> MGHHHHHHSHMAEIGTGFPFDPHYVEVLGERMHYVDVGPRDGTPVLFLHGNPTSSYVWRNIIPHVAPTHRCIAPDLIGMGKS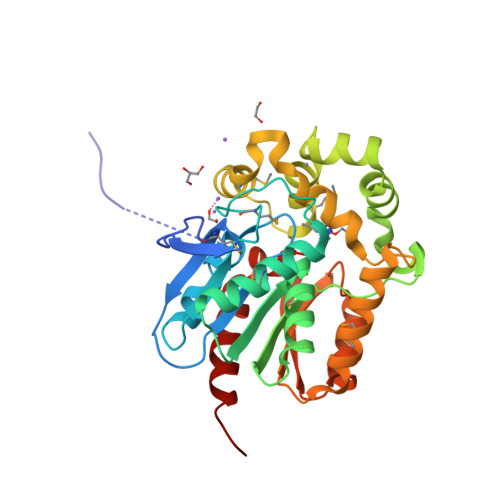DKPDLGYFFDDHVRFMDAFIEALGLEEVVLVIHDWGSALGFHWAKRNPERVKGIAFMEFIRPIPTWDEWPEFARETFQAFRTTDVGRKLIIDQNVFIEGTLPMGVVRPLTEVEMDHYREPFLNPVDREPLWRFPNELPIAGEPANIVALVEEYMDWLHQSPVPKLLFWGTPGVLIPPAEAARLAKSLPNCKAVDIGPGLNLLQEDNPDLIGSEIARWLSTLEISG> SSKMSDVKCTSVVLLSVLQQLRVESSSKLWAQCVQLHNDILLAKDTTEAF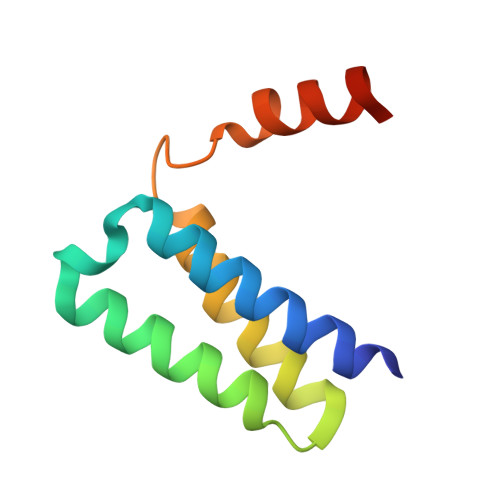EKMVSLLSVLLSMQGAVDINKLCEEMLDNRATLQ>LKCNKLIPLAYKTCPAGKNLCYKMFMVSNKTVPVKRGCIDVCPKNSLLVKYVCCNTD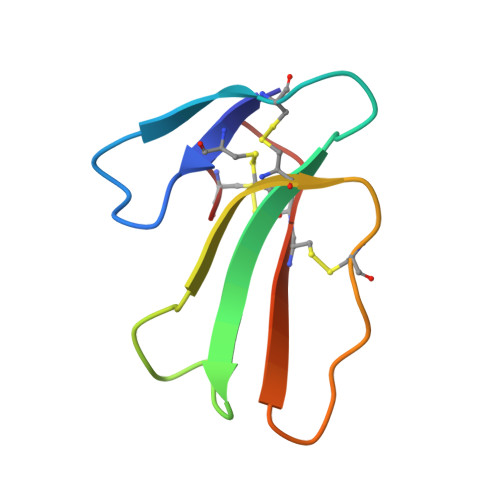RCN[3x]> GSEEDAVDATPLEVFLQSQHLEEFLPIFMREQIDLEALLLCSDEDLQNIHMQLGPRKKVLSAI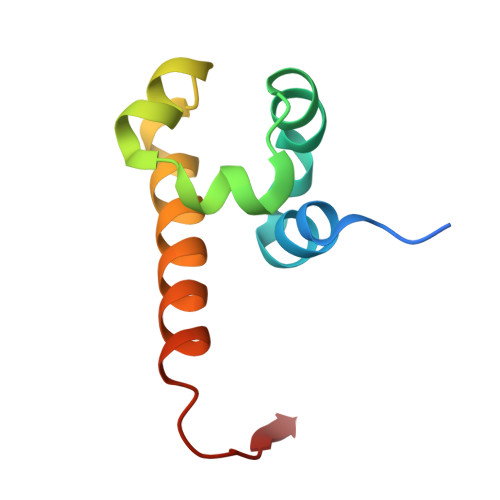DKRKQVLQQPGQLVDTSL> QGEIAIAIPAHVRLVMVANDLPALTDPLVSDVLRALTVSPDQVLQL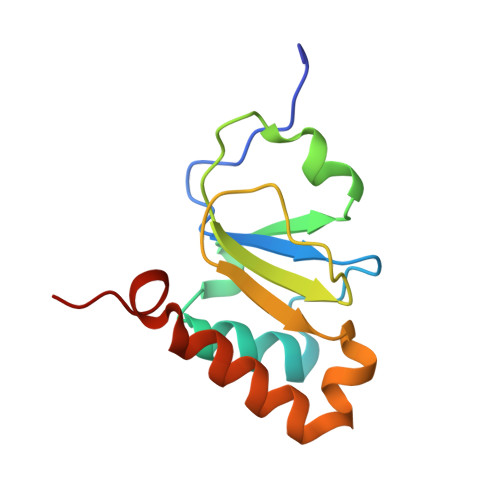TPEKIAMLPQGSHCNSWRLGTDEPLSLEGAQVASPALTDLRANPTARAALWQQICTYEHDFFPRND>MCGIFAYLNYHVPRTRREILETLIKGLQRLEYRGYDSAGVGFDGGNDKDWEANACKIQLIKKKGKVKALDEEVHKQQDMDLDIEFDVHLGIAHTRWATHGEPSPVNSHPQRSDKNNEFIVIHNGIITNYKDLKKFLESKGYDFESETDTETIAKLVKYMYDNRESQDTSFTTLVERVIQQLEGAFALVFKSVHFPGQAVGTRRGSPLLIGVRSEHKLSTDHIPILYRTGKDKKGSCNLSRVDSTTCLFPVEEKAVEYYFASDASAVIEHTNRVIFLE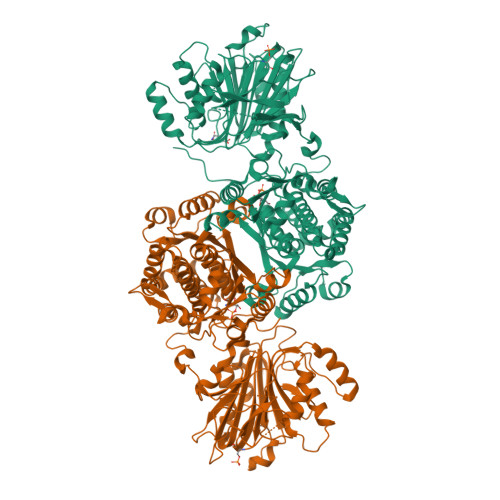DDDVAAVVDGRLSIHRIKRTAGHHHHHHDHPGRAVQTLQMELQQIMKGNFSSFMQKEIFEQPESVVNTMRGRVNFDDYTVNLGGLKDHIKEIQRCRRLILIACGTSYHAGVATRQVLEELTELPVMVELASDFLDRNTPVFRDDVCFFLSQSGETADTLMGLRYCKERGALTVGITNTVGSSISRETDCGVHINAGPEIGVASTKAYTSQFVSLVMFALMMCDDRISMQERRKEIMLGLKRLPDLIKEVLSMDDEIQKLATELYHQKSVLIMGRGYHYATCLEGALKIKEITYMHSEGILAGELKHGPLALVDKLMPVIMIIMRDHTYAKCQNALQQVVARQGRPVVICDKEDTETIKNTKRTIKVPHSVDCLQGILSVIPLQLLAFHLAVLRGYDVDFPRNLAKSVTVE[2x]> MSNKVIYAIYNDDDVLMNAVKKTRAAHHHIEEVFTPFPVHGLDKAMGLAPTRLAICAFLYGCVGISVATTMMSYIMIHDWPQDIGGKPSFSFIQNMPSFVPIM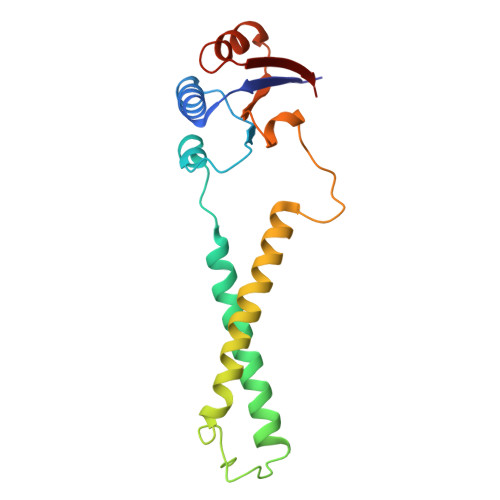FEMTVFFAAHLMVITFYMRSRLWPFKQAENPDVRTTDDHFLIEVAVNDNEAELVSFFEGTGAVEVKVIEKN> MKFLTSNFVQCASKQCV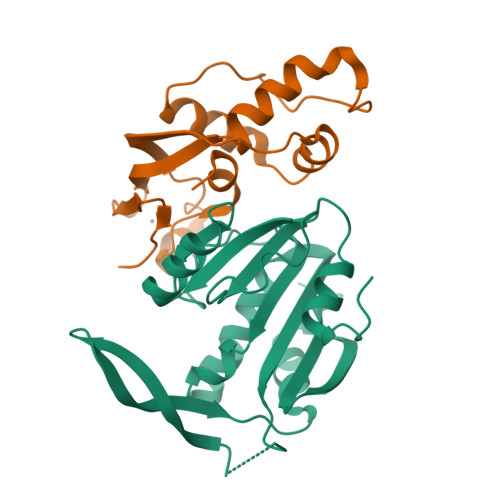SSGNAFPLTFSALEMVQQEAEFDPEFLVSMLERIDWAALVKVANDLGNESLPDVKPEIDEPFAEGNQGLLQELHSLLIETCIVEGTMKCENCGHTYFIKNSIPNFLLPPHLAA;> MANTRYKPWPIVEKFLRDQKDHSVGVDIGCGNGKYMGVNNKVFIVGSDRSDELVKLAHDMDPSREVVVCDAIDNAHPEGRFDFAISIAVIHHFSTPERRREAVRAILNTLRPDGRALIYVWALEQKTSRRGWHEGMDQDVMVPWVKKVDGVEEVRYRYYHLYREGEITSDVEASGGKVLETGYEKDNWWVVAKRGDDWSHHHHHH>TKYPSELIPQMDEWKILLGDGTHKEDLVNYAKDDFFYVEHENETDWVVFKTPNSGITSRTSSNTRTELGQKKHWIPETGGKLNATLKVQHVSTSGDARVAASYSVVVGQIHSDEGHENEPIKIFYKKFPGHTKGSVFWNYEI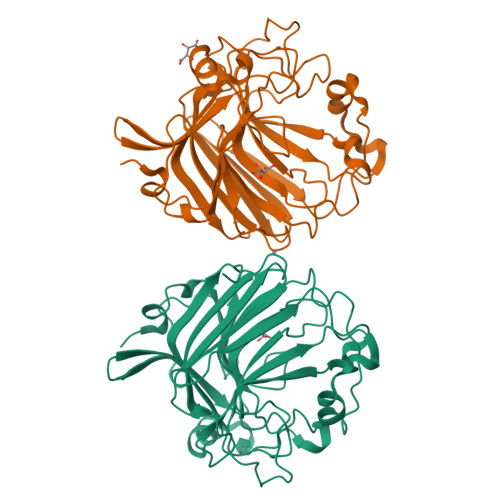NTKGDNSKRWDYSTAVWGYDMSVVGPTATSYPEEPEDGIALGEEFSYEINVYEGIMYLTFSSEGHKTIKFTKNLLKSNFTKKSDIPQQIKTLYASIGRDGIERENAYAGEIQYFKLGAYNQTNGKSPEDNLVWSTGADVYDGDIAKQYANGSYAEVWFKEATLGSGSAPEAQ[2x]> MAEEQPYLEMDLS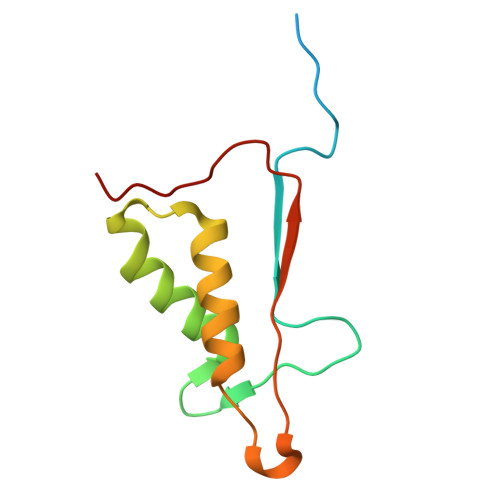SPQTRYIPDEADFLLGMATVNNCVSYRNPAEGTWYIQSLCQSLRERCPRGDDILTILTEVNYEVSNKDDKKNMGKQMPQPTFTLRKKLVFPSD>MRYRPFGSTGVAVSALTLRLADNPRLRANDWRALVFTALENGVNSFQIDGDAPELLKGAGEAFASVERHLLFLTWRLRGDAKQLGPHTLDALKRSAFEGLSLDYLDLLLINDPQSASLPMAFESGLQDLQKGRALRGLGVASRGDIDPGLLANDLVTAVSSPYNLSSGWAERHRIRQASQNNFAVIGEDFWPQALREVADKAPPKPSFWQRRTDPLADVGGYEFLTNTPGWSAEDICLGYALTEPSLATVRVTADNRQEIERLAAVVERD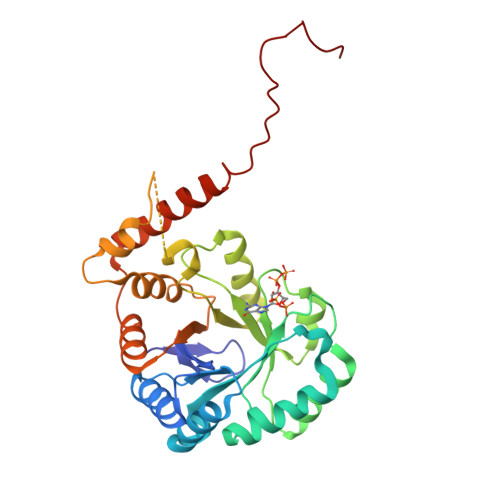LPTGVCAQIEMARFSAQEREKAARRPKLAAALEHHHHHH[4x]> NTWQFKNMISCTVPSRSWWDFADYGCYCGRGGSGTPSDDLDRCCQTHDNCYNEAEKISG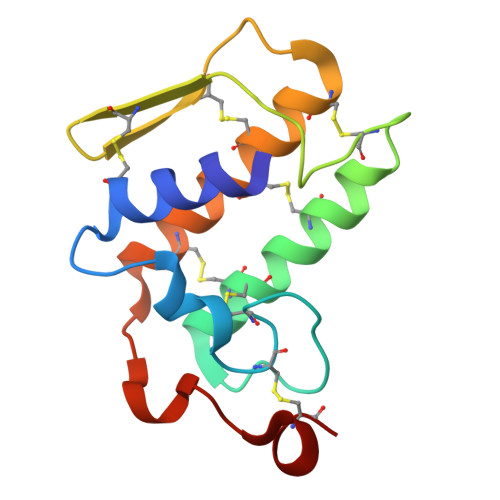CNPRFRTYSYACTAGTLTCTGRNNACAASVCDCDRNAAICFAGAPYNDSNYNIDLQARCN>[2x]MGHHHHHHSHMLAVVGDP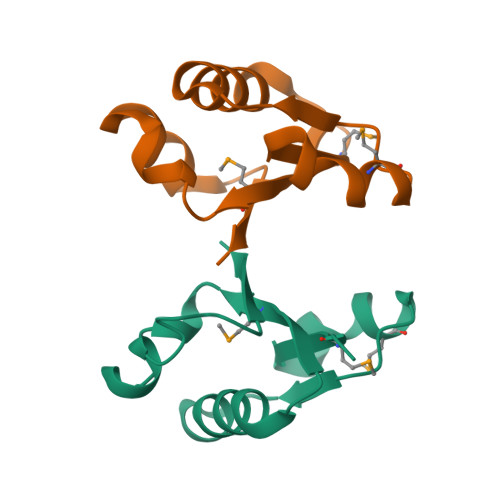DFTIGFMLAGISDIYEVTSDEEIVKAVEDVLKRDDVGVVIMKQEYLKKLPPVLRREIDEKVEPTFVSVGGTGGVEEIREKIRKA> UAGCG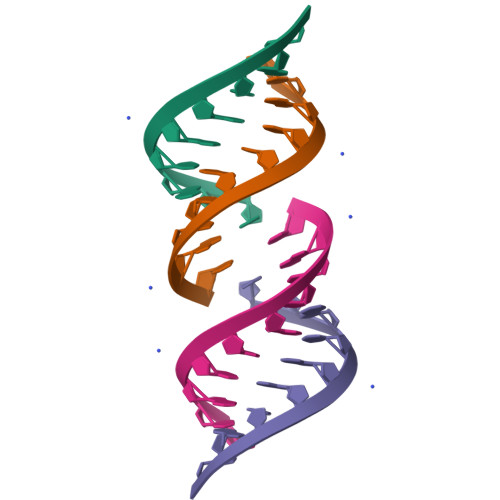GUGC;> GCACCGCUAC;> GCACCGUUGGUAGCGGUGC;> GCACCGCUACCAACGGUGC>FNPCPYSDDTVKMIILTRENKKHDFYTLDTIKKHNEFKKSTIKHQVVFITHGFTSSADTENFLAMAKALSDKGNYLVILIDWRVAACTEEMSGIQLAYYSYAASNTRLVGNYIATVTKMLVQKYNVPMANIRLIGHSLGAHTSGFAGKKVQELGLGKYSEIIGLDPAGPSFKSNDCSERICKTDAHYVQIIHTSNHLGTLVTLGTVDFMNNGYNQPGCGLPLIGETCSHTRAVKYFTECIKHECCLIGVPQSKKPQPVSKCTR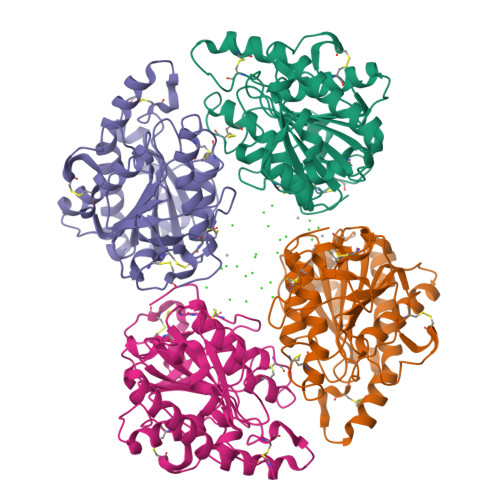NECVCVGLNAKTYPKTGSFYVPVESKAPYCNNKGKII[4x]> CCTGACCAGG;> CCTGGTCAGG

Hairpin pyrrole-imidazole (Py-Im) polyamides can be programmed to bind a broad repertoire of DNA sequences. In addition to targeting the promoter and enhancer regions, our previous results showed that Py-Im induces strong transcriptional arrest of the elongation complex (EC) in a sequence-specific manner, paving the way to target transcription of specific genes. In this study, we solved seven X-ray crystal structures, including a double-stranded DNA complexed with hairpin Py-Im 1 and four different Pol II elongation complexes bound with Py-Im 1. Our structural and functional analyses showed that hairpin Py-Im 1 traps Pol II elongation complex in the n-5 to n-3 position, which forces the elongation complex to be trapped on a futile “treadmill” where Pol II moves back and forth by repetitive extension and cleavage in the presence of TFIIS.

The detailed atomic interaction between hairpin Py-Im 1 and DNA duplex is obscured due to a lack of high-resolution crystal structure of hairpin Py-Im 1 bound with dsDNA complex. Here we obtained a high-resolution crystal structure of the hairpin Py-Im 1–dsDNA (5′-CCTGGTCAGG-3′) complex at 1.8-Å resolution. We observed an intensive hydrogen bonding network that stabilizes the hairpin Py-Im 1–dsDNA complex. Our structure shows the conserved base recognition pattern between Py-Im and DNA base pairs: Im/Py recognizes G/C and Py/Py recognizes A/T or T/A. The binding of hairpin Py-Im 1 leads to minor groove widening as well as major groove compression of the DNA duplex in a similar manner as cyclic Py-Im molecules. In the Py-Im–dsDNA structure, we found that the hydrogen bonding network interactions between the γ-turn moiety of hairpin Py-Im 1 (α-ammonium tip) and the DNA minor groove are mediated by two ordered water molecules.6,8-DIMERCAPTO-OCTANOIC ACID AMIDE | C8 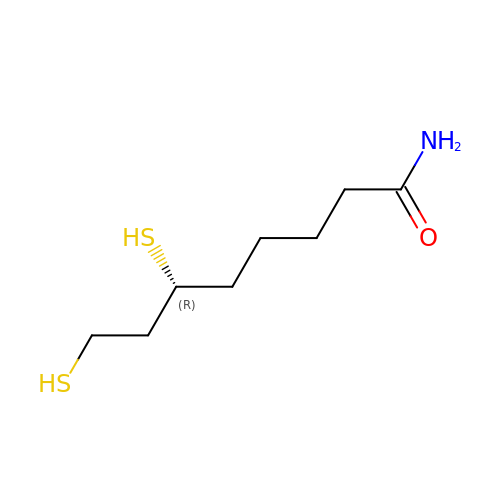H17 N O S2 | VLYUGYAKYZETRF-SSDOTTSWSA-N> MGDKKIVIM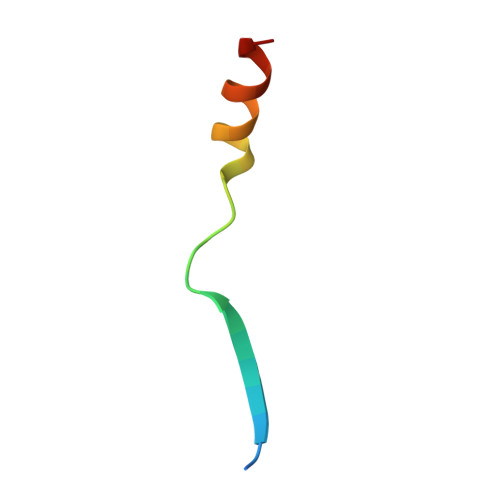PCKCAPSRQLVQVWLQAKE>[2x]MGSLVCVGTGLQLAGQISVLSRSYIEHADIVFSLLPDGFSQRWLTKLNPNVINLQQFYAQNGEVKNRRDTYEQMVNAILDAVRAGKKTVCALFGHPGVFACVSHMAITRAKAEGFSAKMEPGISAEACLWADLGIDPGNSGHQSFEASQFMFFNHVPDPTTHLLLWQIAIAGEHTLTQFHTSSDRLQILVEQLNQWYPLDHEVVIYEAANLPIQAPRIERLPLANLPQAHLMPISTLLIPPAK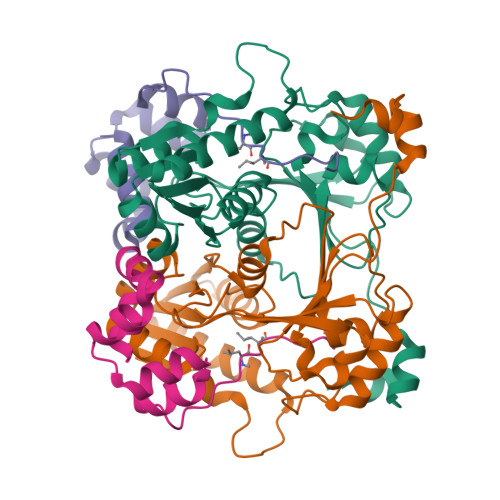KLEYNYAILAKLGIGPEDLG;>[2x]MSGLSDFFTQLGQDAQLMEDYKQNPEAVMRAHGLTDEQINAVMTGDMEKLKTLSGDSSYQSYLVISHGNGD>[6x]MKKQTQLLSALALSVGLTLSASFQAVASIPGQVADQAPLPSLAPMLEKVLPAVVSVRVEGTASQGQKIPEEFKKFFGDDLPDQPAQPFEGLGSGVIINASKGYVLTNNHVINQAQKISIQLNDGRE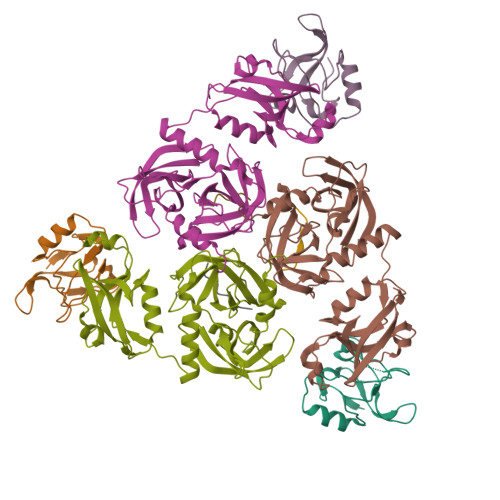FDAKLIGSDDQSDIALLQIQNPSKLTQIAIADSDKLRVGDFAVAVGNPFGLGQTATSGIVSALGRSGLNLEGLENFIQTDASINRGNAGGALLNLNGELIGINTAILAPGGGSVGIGFAIPSNMARTLAQQLIDFGEIKRGLLGIKGTEMSADIAKAFNLDVQRGAFVSEVLPGSGSAKAGVKAGDIITSLNGKPLNSFAELRSRIATTEPGTKVKLGLLRNGKPLEVEVTLDTSTSSSASAEMITPALEGATLSDGQLKDGGKGIKIDEVVKGSPAAQAGLQKDDVIIGVNRDRVNSIAEMRKVLAAKPAIIALQIVRGNESIYLLMRLWHHHHHH> MLRAQKLHSLKSSDITAILPTEQSQKLVLAKKNGDVEVYSRDGNTLKLFQVYPDLLQNAKNDPLPPVIENFYFANELSTIFAQCKETLILLSTTNLHEYDRIIDRRGINHCWLFERSHKNKEE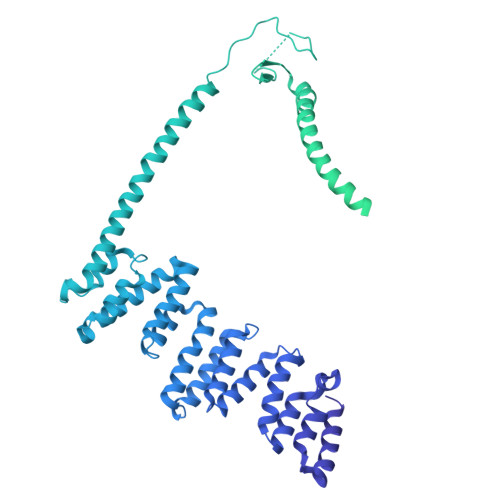KNTYLIYSTINTAKMRVLIWEGRTYKNMMEASLSYRKETIRSIYPGETGITLATDLGIYHWPYNKPSLIRIEKTVKNKFPKDMISALTELKEQAEKVIEKKPKKNSHFDAQSFSSMDRMSRKSSMSSLWYRTIRNERGNKIRYTFELDGNDATPMIIDGATKKIFKVELMHNNEEPFLIATDHATFSESNSEFDHMQYLSSNLLMLYNSSTIKFVDYENGFTFLQQKIPEGIKWVKNLSGTYFLVWTSNDEVQLFSYHVDDGSEDDDQESICGDINDPDFYQLWRKVLFYKFFIDSPHSKELCVSDNPEESLDICAMKLRDLTVMWCLRIFDKFQNYMVQLERSRNSRMIRSKCEEMIIKSIFDLFIKFWAPPQLVILKVFPSAISSLVLEITGQEHHCLLKEAEEVKETYDIPPHLLNRWCLPYLTDTRRHLQNLLSKENDDESRITWCYRDREIKQSFDFFLISNHDDVDLNTMLTLIDTVLFKCYLYYNPPMVGPFIRVENHCDSHVIVTELKIRHMFKDLIDFYYKRGNHEEALKFLTDLVDELENDNTDQKQRQKIDHGVKILVIYYLKKLSNPQLDVIFTYTDWLLNRHNDSIKEILSSIFFYDSQACSSRDHLKVYGYIKKFDKLLAIQYLEFAISTFRLEGNKLHTVLIKLYLENLDIPSTRIKLKSLLETTSVYEPRTILKLLNDAIESGSDQLPTNQLNFVKYLKIFPLSKLENHKEAVHILLDEIDDYKAATSYCNDVYQSDSTKGEELLLYLYSKLVSIYDSNRNSKLILNFLQDHGSKLNSAEIYKNLPQDISLYDIGRVVSQLLKKHTSKMDETRLEKALLQVELVATTYKLNERMSSYGVLSDSHKCPICKKVISNFGTDSISWFTREGRNIITHYNCGKVLQERFNAKNEKSSRIKQKTLGEVINELNNK>MEEGFRDRAAFIRGAKDIAKEVKKHAAKKVVKGLDRVQDEYSRRSYSRFEEEDDDDDFPAPSDGYYRGEGTQDEEEGGASSDATEGHDEDDEIYEGEYQGIPRAESGGKGERMADGAPLAGVRGGLSDGEGPPGGRGEAQRRKEREELAQQYEAILRECGHGRFQWTLYFVLGLALMADGVEVFVVGFVLPSAEKDMCLSDSNKGMLGLIVYLGMMVGAFLWGGLADRLGRRQCLLISLSVNSVFAFFSSFVQGYGTFLFCRLLSGVGIGGSIPIVFSYFSEFLAQEKRGEHLSWLCMFWMIGGVYAAAMAWAIIPHYGWSFQMGSAYQFHSWRVFVLVCAFPSVFAIGALTTQPESPRFFLENGKHDEAWMVLKQVHDTNMRAKGHPERVFSVTHIKTIHQEDELIEIQSDTGTWYQRWGVRALSLGGQVWGNFLSCFGPEYRRITLMMMGVWFTMSFSYYGLTVWFPDMIRHLQAVDYASRTKVFPGERVEHVTFNFTLENQIHRGGQYFNDKFIGLRLKSVSFEDSLFEECYFEDVTSSNTFFRNCTFINTVFYNTDLFEYKFVNSRLINSTFLHNKEGCPLDVTGTGEGAYMVYFVSFLGTLAVLPGNIVSALLMDKIGRLRMLAGSSVMSCVSCFFLSFGNSESAMIALLCLFGGVSIASWNALDVLTVELYPSDKRTTAFGFLNALCKLAAVLGISIFTSFVGITKAAPILFASAALALGSSLALKLPSRLEEELRRRTEPGSLEVLFQ[2x]

Synaptic vesicle glycoprotein 2A (SV2A) represents a novel antiepileptic targeted by the prescribed levetiracetam (LEV, Keppra®) and brivaracetam (BRV, BRIVIACT®). SV2 proteins are critical to neuromodulation and neurotransmission, and a well-established role of SV2 is as a crucial regulator of synaptotagmin trafficking. SV2A protein is predicted to share structural similarity with the major facilitator superfamily (MFS) transporters; however, it is not classified into any existing solute carrier (SLC) family. The overall SV2A architecture can be divided into three parts: the intracellular helical domain (IHD), the transmembrane domain (TMD), and the glycosylated luminal quadrilateral β-helix domain (LBD).

2D classification revealed that SV2A protein existed in both monomeric and dimeric states, in the absence of any ligand (apo). However, we could not reconstruct the monomeric map due to relatively weak signals; instead, we determined the dimeric structure at 3.5 Å resolution (dubbed as SV2AApo), with C1 symmetry. Intriguingly, no obvious opening is available on either the cytosol or the lumen side of SV2AApo TMD, indicating an occluded state captured for the SV2AApo structure. Roughly related by a two-fold pseudosymmetry, the two protomers of the dimeric SV2AApo are superimposed with a Cα root mean square deviation (RMSD) of 0.9 Å. However, they are not identical, in particular the TMDs, which show significant variation. For one protomer, the typical MFS-fold 12-transmembrane helices were built into the EM density of higher resolution, referred to as the canonical form (C-form). In contrast, only 11 TMs could be modeled for the other protomer, due to the lack of TM12 density. Furthermore, the peripheral TM9 swung away from the TMD core, instead of packing against TMs 7, 10, and 12 as seen in the C-form, to engage with the neighboring TM8 of the C-form protomer. We defined the configuration of this unusual protomer as a non-canonical variant (NC-form). The dimeric interface was mainly formed between TMs 8 and 10, with additional contribution from TM9 of the NC-form protomer.>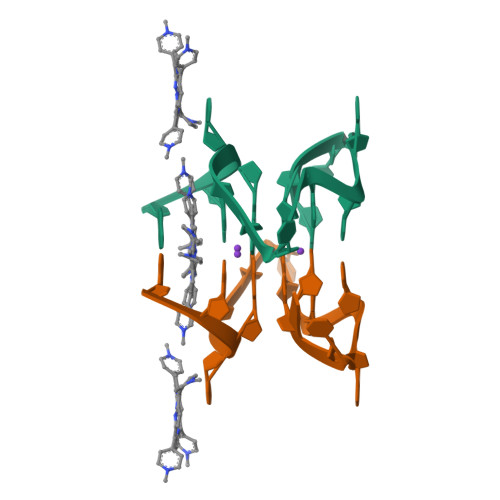 GGCUCGGCGGCGGA>MAQTLLSSFGTPFERVENALAALREGRGVMVLDDEDRENEGDMIFPAETMTVEQMALTIRHGSGIVCLCITEDRRKQLDLPMMVENNTSAYGTGFTVTIEAAEGVTTGVSAADRITTVRAAIADGAKPSDLNRPGHVFPLRAQAGGVLTRGGHTEATIDLMTLAGFKPAGVLCELTNDDGTMARAPECIEFANKHNMALVTIEDLVAYRQAHERKA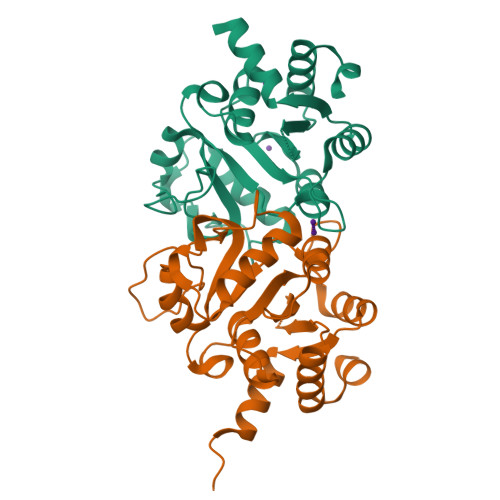S[2x]>[2x]MADPAECSIKVMCRFRPLNEAEILRGDKFIPKFKGEETVVIGQGKPYVFDRVLPPNTTQEQVYNACAKQIVKDVLEGYNGTIFAYGQTSSGKTHTMEGKLHDPQLMGIIPRIAHDIFDHIYSMDENLEFHIKVSYFEIYLDKIRDLLDVSKTNLAVHEDKNRVPYVKGCTERFVSSP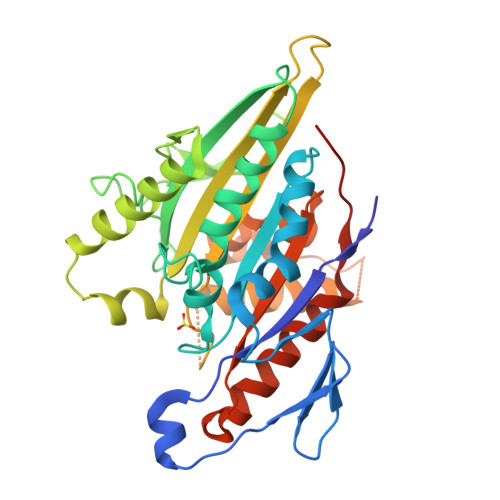EEVMDVIDEGKANRHVAVTNMNEHSSRSHSIFLINIKQENVETEKKLSGKLYLVDLAGSEKVSKTGAEGAVLDEAKNINKSLSALGNVISALAEGTKTHVPYRDSKMTRILQDSLGGNCRTTIVICCSPSVFNEAETKSTLMFGQRAKTIKNTVSVNHHHHHHH> GPH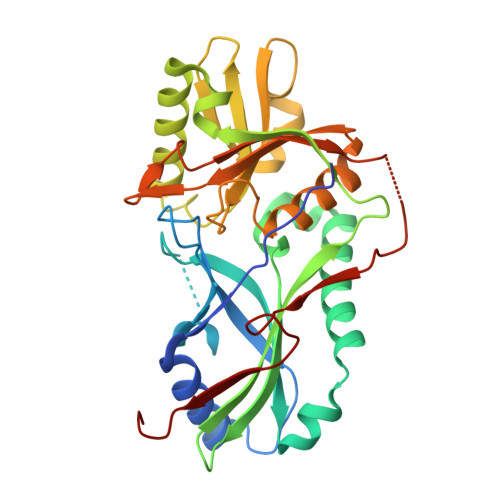MPAIILQFAPLNSSVDEGFWHSFSSLKLDKLGIDDSPISITGFYGPCGHPQVSNHLTLLSESLPLDEQSLIASTSHGNRNKCPVPGILYNTNTVESFNKLDKQSLLKAEANKIWEDIQSGKALEDPSVLPRFLVISFADLKKWSFRYWFAFPAFVLDPPVSLIELKPASEYFSSEEAESVSAACNDWRDSDLTTDVPFFLVSVSSDSKASIRHLKDLEACQGDHQKLLFGFYDPCHLPSNPGWPLRNYLALIRSRWNLETVWFFCYRESRGFADLNLSLVGQASITLSSGESAETVPNSVGWELNKGKRVPRSISLANSM> LT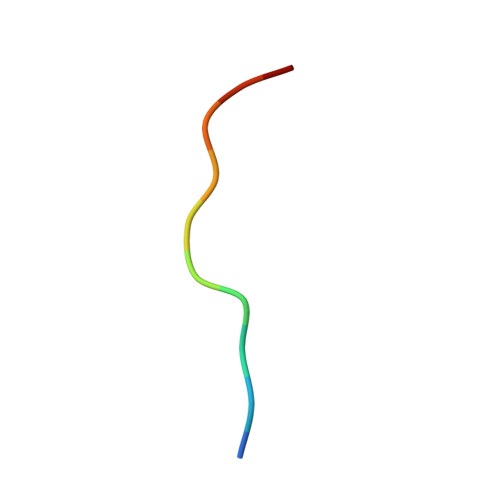GCGDIIAEQ>AVSKVYARSVYDSRGNPTVEVELTTEKGVFRSIVPSGAATGVHEALEMRDGDKSKWMGKGVLHAVKNVNDVIAPAFVKANIDVKDQKAVDDFLISLDGTANKSKLGANAILGVSLAASRAAAAEKNVPLYKHLADLSKSKTSPYVLPVPFLNVLNGGSHAGGALALQEFMIAPTGAKTFAEALRIGSEVYHNLKSLTKKRYGASAGNVGDEGGVAPNIQTAEEALDLIVDAIKAAGHDGKIKIGLDCASSEFFKDGKYDLDFKNPNSDKSKWLTGPQLADLYHSLMKRYPIVSIEDPFAEDDWEAWSHFFKTAGIQIVADALTVTNPKRIATAIEKKAADALLLKVNQ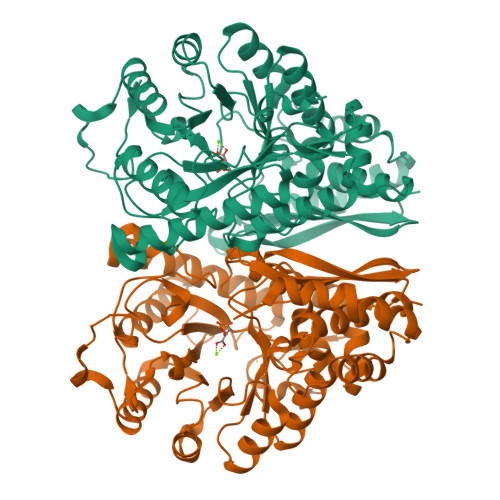IGTLSESIKAAQDSFAAGWGVMVSHRSGETEDTFIADLVVGLRTGQIKTGAPARSERLAKLNQLLRIEEELGDNAVFAGENFHHGDKLLHHHHHH[4x]5-cyclopropyl-1H-imidazol-2-amine 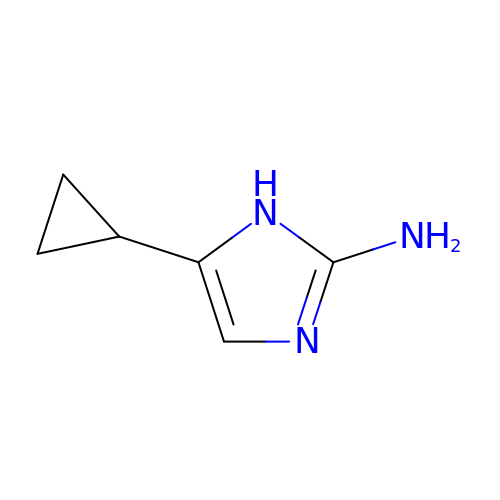| C6 H9 N3 | LHDVWRMWQJIACV-UHFFFAOYSA-N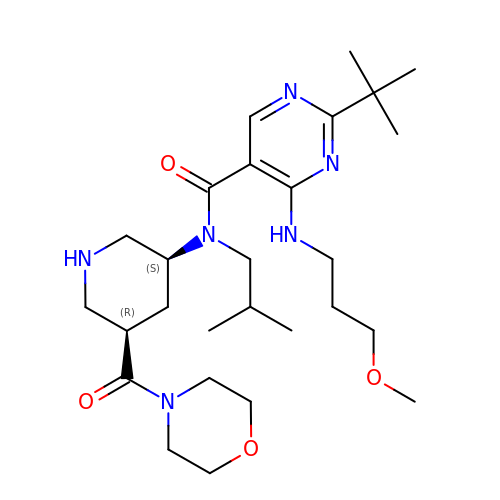2-~{tert}-butyl-4-(3-methoxypropylamino)-~{N}-(2-methylpropyl)-~{N}-[(3~{S},5~{R})-5-morpholin-4-ylcarbonylpiperidin-3-yl]pyrimidine-5-carboxamide | C27 H46 N6 O4 | ISBMTDVOSWIALV-RTWAWAEBSA-N> SLVMSSPALPAFLLCSTLLVIKMYVVAIITGQVRLRKKAFANPEDALRHGGPQYCRSDPDVERCLRAHRNDMETIYPFLFLGFVYSFLGPNPFVAWMHFLV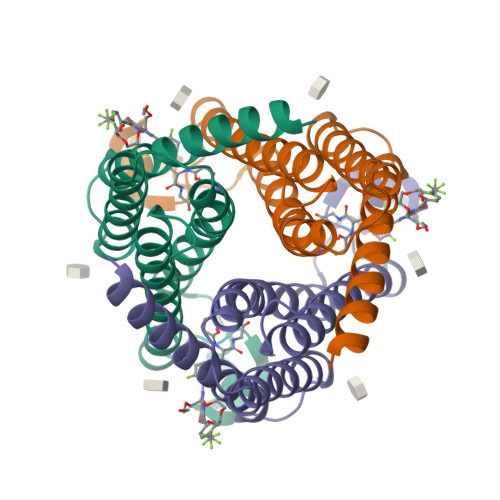FLVGRVAHTVAYLGKLRAPIRSVTYTLAQLPCASMALQILWEAARHL>[2x]MSKVPSDIEIAQAAKMKPVMELARGLGIQEDEVELYGKYKAKISLDVYRRLKDKPDGKLILVTAITPTPAGEGKTTTSVGLTDALARLGKRVMVCLREPSLGPSFGIKGGAAGGGYAQVVPMEDINLHFTGDIHAVTYAHNLLAAMVDNHLQQGNVLNIDPRTITWRRVIDLNERALRNIVIGLGGKANGVPRE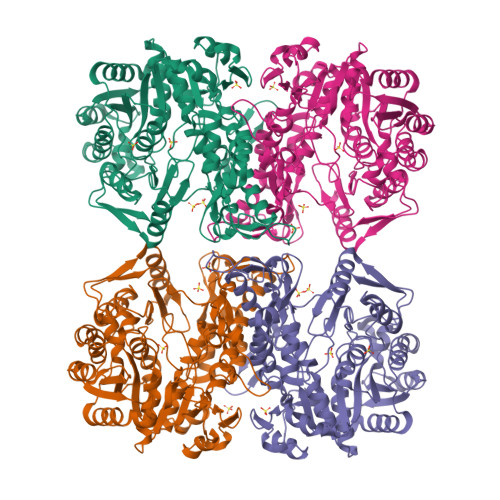TGFDISVASEVMACLCLASDLMDLKERFSRKVVGYTYDGKPVTAGDLEAQGSMALLMKDAIKPNLVQTLENTPAFIHGGPFANIAHGCNSIIATKTALKLADYVVTEAGFGADLGAEKFYDVKCRYAGFKPDATVIVATVRALKMHGGVPKSDLATENLEALREGFANLEKHIENIGKFGVPAVVAINAFPTDTEAELNLLYELCAKAGAEVALSWAKGGEGGLELARKVLQTLESRPSNFHVLYNLDLSIKDKIAKIATEIYGADGVNYTAEADKAIQRYESLGYGNLPVVMAKTQYSFSDDMTKLGRPRNFTITVREVRLSAGGRLIVPITGAIMTMPGLPKRPAACNIDIDADGVITGLF>[12x]ATYFTYYSA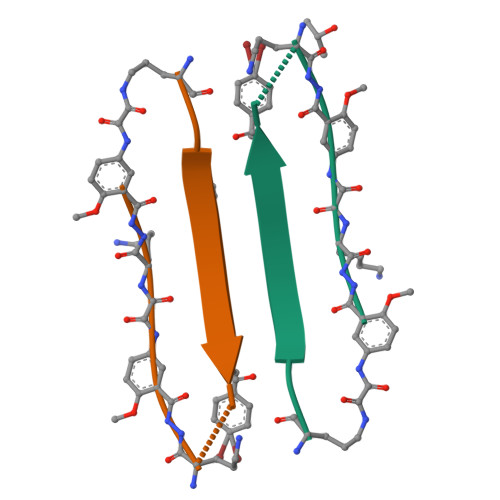XKX>MITVDITVNDEGKVTDVIMDGHADHGEYGHDIVSAGASAVLFGSVNAIIGLTSERPDINYDDQGGHFHIRSVDTNNDEAQLILQTMLVSLQTIEE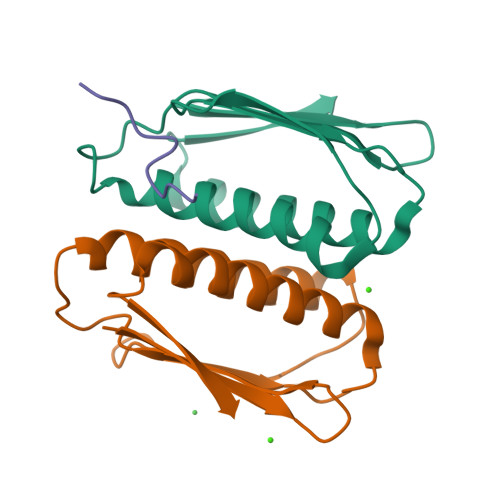EYNENIRLNYK[2x];> XKLNLQFFASKKGX>[4x]SNAMKI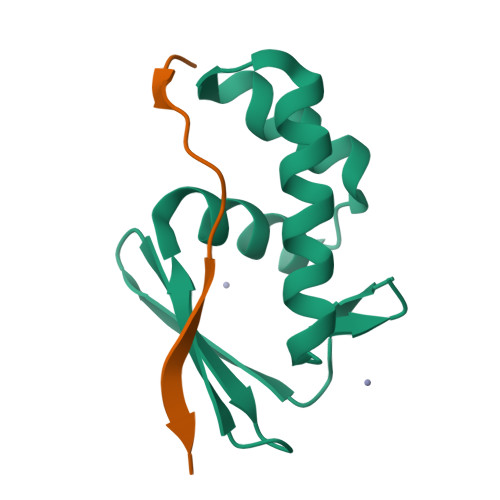SDAVVSAHIDDEVVLLHLQTGTYFGLDAVGSRIWSLLEEGKRPEEIVDAICAEYSVDRPTVERDLRDFLRALANKELLEGYADEA;>[4x]MTKTYTAPTLVEYGGLERLT>VPTLQRDVAIVGAGPSGLAAATALRKAGLSVAVIEARDRVGGRTWTDTIDGAVLEIGGQWVSPDQTALISLLDELGLKTFERYREGESVYISSAGERTRYTGDSFPTNETTKKEMDRLIDEMDDLAAQIGAEEPWAHPLARDLDTVSFKQWLINQSDDAEARDNIGLFIAGGMLTKPAHSFSALQAVLMAASAGSFSHLVDEDFILDKRVIGGMQQVSIRMAEALGDDVFLNAPVRTVKWNESGATVLADGDIRVEASRVILAVPPNLYSRISYDPPLPRRQHQMHQHQSLGLVIKVHAVYETPFWREDGLSGTGFGASEVVQEVYDNTNHEDDRGTLVAFVSDEKADAMFELSAEERKATILASLARYLGPKAEEPVVYYES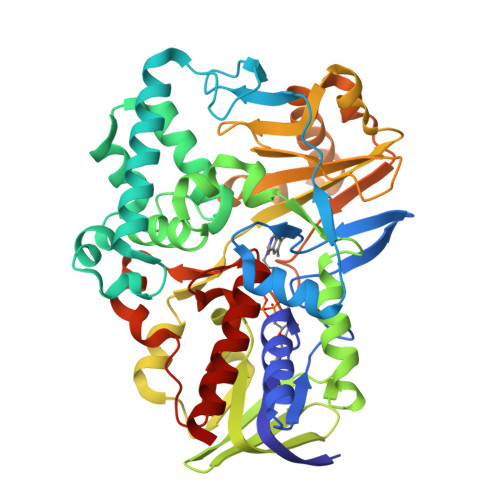DWGSEEWTRGCYTASFDLGGLHRYGADSRTPVGPIHFSCSDIAAEGYGHVDGAVRMGQRTAADIIARSKA[2x]>[4x]KEAETQQKLANVVILATGGTIAGAGASAANSATYQAAKLGVDKLIAGVPELADIANVRGEQVMQIASESISNDDLLKLGKRVAELAESKDVDGIVITHGTDTLEETAFFLNLVEKTDKPIVVVGSMRPGTAMSADGMLNLYNAVAVASDKQSRGKGVLVTMNDEIQSGRDVSMAVNIKTEAFKSAWGPM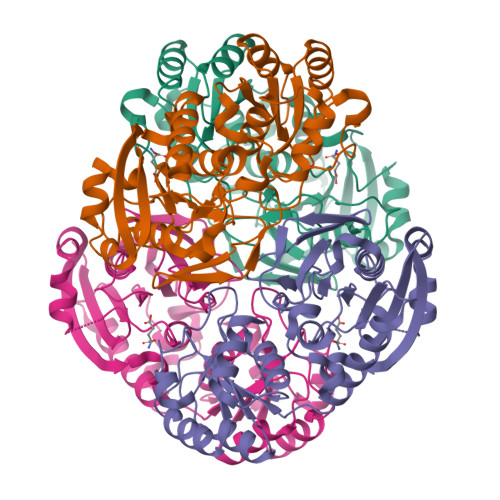GMVVEGKSYWFRLPAKRHTVNSEFDIKQISSLPQVDIAYGYGNVTDTAYKALAQNGAKALIHAGTGNGSVSSRVVPALQELRKNGVQIIRSSHVNQGGFVLRNAEQPDDKNDWVVAHDLNPQKARILAMVAMTKTQDSKELQRIFWEY> VPATRILLLVLAVIIYGTAGFHFIEGESWTVSLYWTFVTIATVGYGDYSPSTPLGMYFTVTLIVL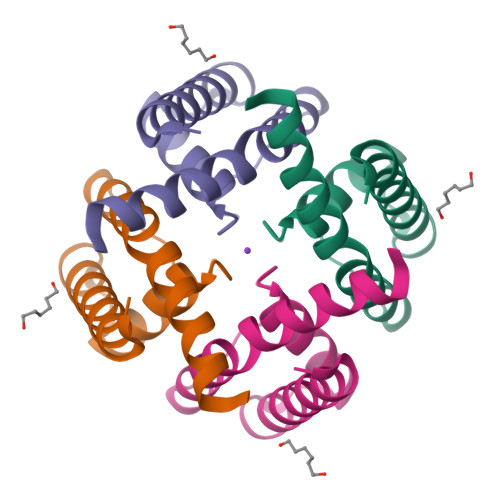GIGTFAVAVERLLEFLI>GTKQEKTALNMARFIRSQTLTLLEKLNELDADEQADICESLHDHADELYRSC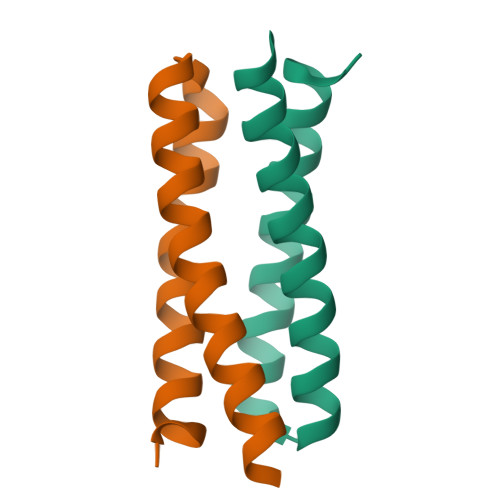LARFGDDGENL[2x]> CPDACCPHGSSGLRCTRDGALDSLHHLPGAENLTELYIENQQHLQHLELRDLRGLGELRNLTIVKSGLRFVA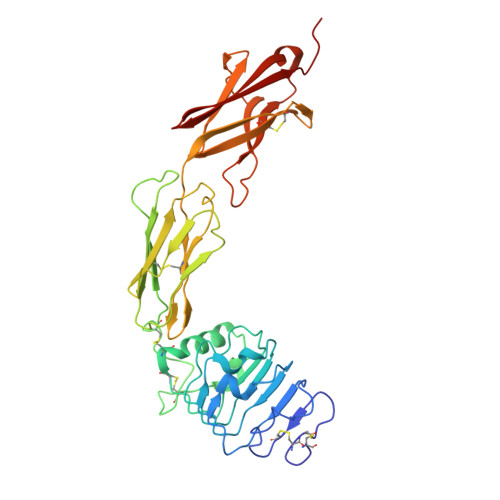PDAFHFTPRLSRLNLSFNALESLSWKTVQGLSLQELVLSGNPLHCSCALRWLQRWEEEGLGGVPEQKLQCHGQGPLAHMPNASCGVPTLKVQVPNASVDVGDDVLLRCQVEGRGLEQAGWILTELEQSATVMKSGGLPSLGLTLANVTSDLNRKNVTCWAENDVGRAEVSVQVNVSFPASVQLHTAVEMHHWCIPFSVDGQPAPSLRWLFNGSVLNETSFIFTEFLEPAANETVRHGCLRLNQPTHVNNGNYTLLAANPFGQASASIMAAFMDNP Banna virus (BAV) is the prototype Seadornavirus, a class of reoviruses for which there has been little structural study. Here, we report atomic cryo-EM structures of three states of BAV virions—surrounded by 120 spikes (full virions), 60 spikes (partial virions), or no spikes (cores). In the full and partial BAV virions, genomic dsRNA segments and a number of RNA-dependent RNA polymerases (RdRps, VP1) are packaged in a double-layered icosahedral capsid consisting of three proteins (VP2, VP8, and VP10). The spikes protruding from the outer capsid shell are heterohexamers composed of a VP4 trimer capped by a VP9 trimer.

The C5 reconstruction focusing on vertices of full particles revealed only low-resolution density for VP9, except the N-terminal fragment containing one α-helix, reflecting structural variations in the head domains of the VP9 trimer relative to the N-terminal α-helices. The α1-helices from the three protomers form a tripod-like conformation, which is situated in a central cavity surrounded by pedestal domains of the VP4 trimer. Residues from the unfurling domain (D71, S74, and D78) and the pedestal domain (K466, D499, T500, N502, E503, Q525, and K565) of VP4 form hydrogen bonds with residues from the tripod to anchor the VP9 trimer onto the VP4 trimer. A density map of the VP9 trimer at an overall resolution of 3.8 Å was obtained by iterative 3D classifications and subpopulation averaging of the VP9 density at multiple positions, allowing us to resolve an atomic model for almost full-length VP9 (covering residues 4–283). The VP9 stalk adopts a helix–loop–helix–loop–helix conformation, and multiple residues are involved in interprotomer interactions. The extended loops connecting helices α1 and α2 serve as the internal hinge for tilting of the C-terminal parts of VP9 trimers. Considering the large number of VP9 trimers on the BAV particles, the structural plasticity of loops in the stalk region of VP9 may facilitate the interactions of rigid head domains with multiple receptor molecules on host cells with variable binding orientations. The viral infection is initiated by VP9, which recognizes and attaches to unknown cellular receptors in a multivalent-binding manner.

>[3x]MLSETELRALKKLSTTTSRVVGDSTLALPSNVKLSKGEVEKIAVTKKEMFDELAQCNLPTIELITREHTFNGDVIRFAAWLFLMNGQKLMIANNVAVRMGMQYATNLAGNNVKITYVTSNNVVKLGHIAAGVLANPYSNKGSGLFITYEYNLISNLIETGKVCVLFITSLSTTASSTNSFAYSTCSVPIENWDFNMIKLTAETSCASLTAMTNLVNSLVPGERTRPVGLYVDIPGVTVTTSASSGSLPLTTIPAVTPLIFSAYTKQVEEVGVINTLYALSYLP>[2x]GSHMKNVLIGVQTNLGVNKTGTEFGPDDLIQAYPDTFDEMELISVERQKEDFNDKKLKFKNTVLDTCEKIAKRVNEAVIDGYRPILVGGDHSISLGSVSGVSLEKEIGVLWISAHGDMNTPESTLTGNIHGMPLALLQGLGDRELVNCFYEGAKLDSRNIVIFGAREIEVEERKIIEKTGVKIVYYDDILRKGIDNVLDEVKDYLKIDNLHISIDMNVFDPEI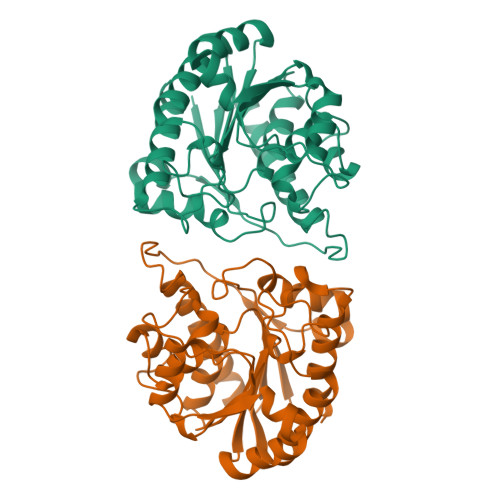APGVSVPVRRGMSYDEMFKSLKFAFKNYSVTSADITEFNPLNDINGKTAELVNGIVQYMMNPDY>MKDCSNGCSAECTGEGGSKEVVGTFKAKDLIVTPATILKEKPDPNNLVFGTVFTDHMLTVEWSSEFGWEKPHIKPLQNLSLHPGSSALHYAVELFEGLKAFRGVDNKIRLFQPNLNMDRMYRSAVRATLPVFDKEELLECIQQLVKLDQEWVPYSTSASLYIRPTFIGTEPSLGVKKPTKALLFVLLSPVGPYFSSGTFNPVSLWANPKYVRAWKGGTGDCKMGGNYGSSLFAQCEAVDNGCQQVLWLYGEDHQITEVGTMNLFLYWINEDGEEELATPPLDGIILPGVTRRCILDLAHQWGEFKVSERYLTMDDLTTALEGNRVREMFGS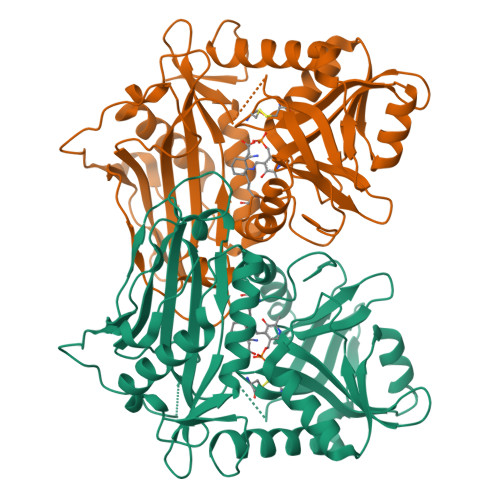GTACVVCPVSDILYKGETIHIPTMENGPKLASRILSKLTDIQYGREERDWTIVLS[2x]> MAIKVIEEKCIGCSKCQKSCPFD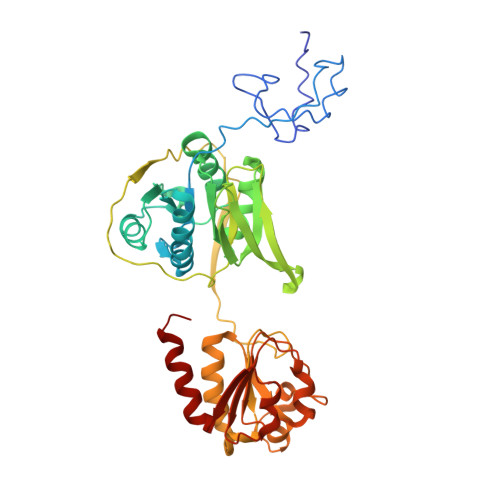AITIENKIAVIGDACTNCGTCIDVCPTEAILQEGTEKIVRDLSMYKGVWVFAEQREGKIMPVVFELLGEGKKLANEIGTELCAILCGSNVAELTDELFAYGADKVYLADAPELEKYTTDGYSKIINEAIGLYKPEIVLYGATHIGRDLAPCLAVKVNTGLTADCTKLEIDPDDKKIRQTRPAFGGNLMATIVCPGSRPQMSTVRPGVMDKAAYDPSQKGEVIKLDATFNEGDIRTKVLEIVKTTTDNISISDADFIVSGGMGLGKPEGFELLKQLADKLGGTVATSRACVDAGWADHAQQVGQTGTTVKPQIYFACGISGAIQHIAGMQDSDIIIAINKNENAPIFEVADYGIVGDLYKVIPAIIEELDKIGK> TFTAKTGTNFGNDNDAEAYLQFEKLIDKKYLKLPTRVNLEILRGTKIHSSFLFNSYSSLSPQSILNLKVFSQFYNWNTNKGLDIGQRGARLSLRYEPLFLHKLLHNPHSNESPTLFHEWFLETCWRSTKICSQGTSAPYMYSGTMLSQAGDQLRTILGHTFVLDKRDHIMCPTK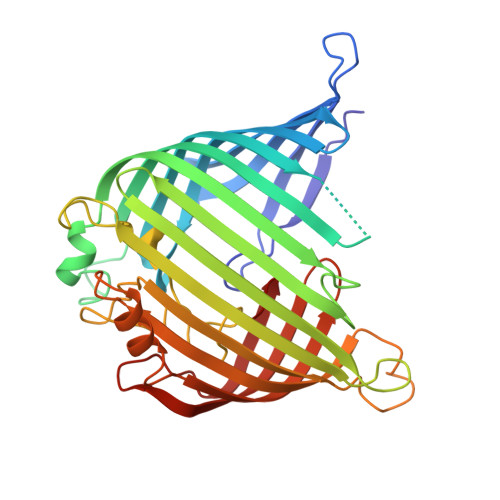GSMLKWSNELSPGKHLKTQLELNSVKSWMNDDFITFSTTIKTGYLKNLSSQQSLPVHICDKFQSGGPSDIRGFQTFGLGPRDLYDAVGGDAFVSYGLSVFSRLPWKKVEKSNFRLHWFFNGGKLVNHDNTSLGNCIGQLSKEHSTSTGIGLVLRHPMARFELNFTLPITAHENDLIRKGFQFGLGLAFL> MSKLDLHQMTTQDLVALFAKVTVEQDDALLGNQISRFNRLFGVMAEIADELKARDGDQRTALLSLFEYPN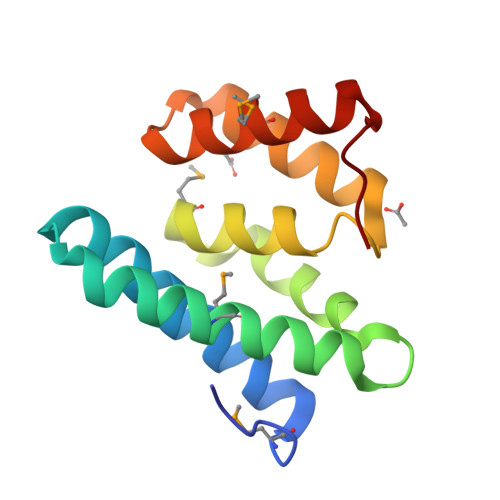MQVRLQAAKLTLAVAPVKAREQLEAIVSSKWFPQAGDAGMCLDLLDDGTFKPK> GMGGAALPDNGWPADRIDTESAHSARIYDYIIGGKDYYPADKEAGDAMSREWPALPVHMRANRDWMNRAVAHLAKEAGIRQFLDIGTGIP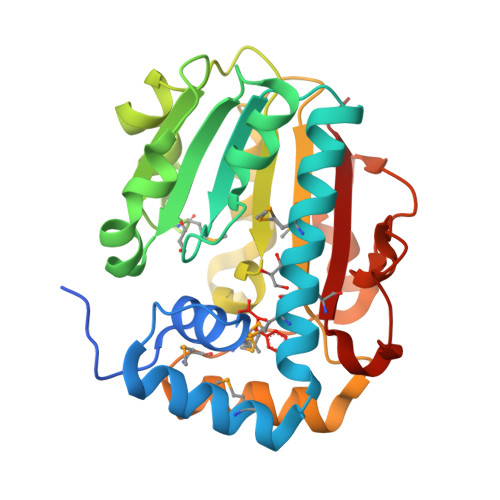TSPNLHEIAQSVAPESRVVYVDNDPIVLTLSQGLLASTPEGRTAYVEADMLDPASILDAPELRDTLDLTRPVALTVIAIVHFVLDEDDAVGIVRRLLEPLPSGSYLAMSIGTAEFAPQEVGRVAREYAARNMPMRLRTHAEAEEFFEGLELVEPGIVQVHKWHPDAATADGIRDEDIAMYGAVARKP>[2x]GAMNAQAEEFKKYLETNGIKPKQFHKKELIFNQ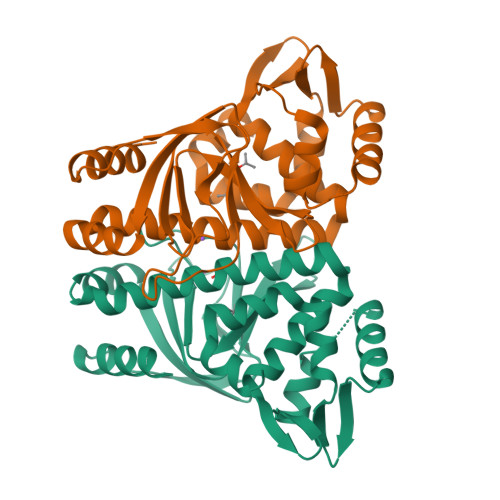WDPQEYCIFLYDGITKLTSISENGTIMNLQYYKGAFVIMSGFIDTETSVGYYNLEVISEQATAYVIKINELKELLSKNLTHFFYVFQTLQKQVSYSLAKFNDFSINGKLGSICGQLLILTYVYGKETPDGIKITLDNLTMQELGYSSGIAHSSAVSRIISKLKQEKVIVYKNSCFYVQNLDYLKRYGPKLDEWFYLACPATWGKLN>MQWSGARALEALLTVAGELRGPPLQLDTGQLLKIAKRGGVTAVEAVHAWRNALTGAPLNLTPEQVVAIASHDGGKQALETVQRLLPVLCQAHGLTPQQVVAIASHDGGKQALETVQRLLPVLCQAHGLTPEQVVAIASNSGGKQALETVQALLPVLCQAHGLTPEQVVAIASNSGGKQALETVQRLLPVLCQAHGLTPQQVVAIASHDGGKQALETVQRLLPVLCQAHGLTPQQVVAIASNGGGKQALETVQRLLPVLCQAHGLTPQQVVAIASNSGGKQALETVQRLLPVLCQAHGLTPQQVVAIASHDGGKQALETVQRLLPVLCQAHGLTPQQVVAIASNGGGKQALETVQRLLPVLCQAHGLTPEQVVAIASNSGGKQALETVQRLLPVLCQAHGLTPEQVVAIASNNGGKQALETVQRLLPVLCQAHGLTPQQVVAIASNSGGRPALESIVAQLSRPDPALAALTNDHLVALACLGGRPALDAVKKLEHHHHHH[2x]

Transcription activator-like (TAL) effectors specifically bind to double stranded (ds) DNA through a central domain of tandem repeats. Each TAL effector (TALE) repeat comprises 33–35 amino acids and recognizes one specific DNA base through a highly variable residue at a fixed position in the repeat. The crystal structures of TAL effector (TALE) proteins bound to their respective target DNAs have revealed that the residue at position 13 is the only one directly involved in DNA base recognition, whereas the 12th residue stabilizes the proper loop conformation. dHax3, an engineered TALE protein, proved to be a useful scaffold for structural characterizations. We then present fifteen crystal structures of engineered dHax3 variants in complex with target DNA molecules, which elucidate the structural basis for the recognition of bases adenine (A) and guanine (G) by reported or uncharacterized TALE codes.

As a proof-of-principle, we generated two dHax3 variants, dHax3-NI, in which Ile34 was introduced at repeat 7 to replace Ser34 for recognition of base A, and dTALE (standing for designed TALE repeats), in which the RVDs in repeats 3–12 were replaced and the protein recognize an artificial DNA element (5′-TCCAACTACTAGA-3′). Two structures were determined for DNA-bound dHax3-NI at 2.8 Å and 2.2 Å, respectively. The structure of dTALE in complex with the target DNA element was refined at 2.4 Å resolution. The structures of DNA-bound dTALE can be superimposed to dHax3 with an RMSD (root-mean-squared deviation) of 0.946 Å over 455 Cα atoms with the major deviation occurring to the amino (N) terminal helix. Similarly, structural comparison of DNA-bound dHax3 and PthXo1 reveals an RMSD of 1.04 Å over 429 Cα atoms. These observations corroborated the notion that DNA binding by TALE repeats is modular and context free. While the coordination of base A by Ile34 is almost identical in the structures of dHax3-NI and PthXo1, the binding of base G by dTALE shows some subtle but important difference. In the PthXo1-DNA complex structure, Asn34 is hydrogen-bonded (H-bonded) to the N7 atom of base G; in the high-resolution structure of dTALE, however, the side group of Asn34 donates a H-bond to O6 atom of G. Given that O6 atom is more electronegative than N7 atom in base G, the H-bond with O6 atom may represent a stronger interaction. Asn34 form the hydrogen bond in a different way with both A and G. The length of the hydrogen bonds are about 3 Å.>MAGAIKVGTWGGNGGSEWDMGPAYRIDSVKINAGDIIDAIEITFTRYGLTETQHYGGTGGEPHEIAFEDGEYIMSMEGHVVDYTGLTIIGK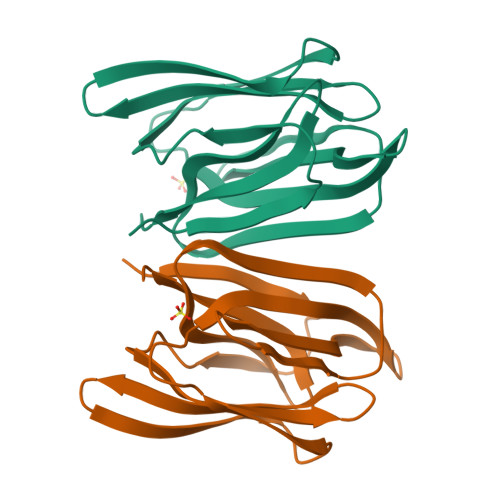LTLTTNRRTFGPFGAYEGTPFSIPVAEGKIAGFFGRAGSFIDAIGVYLMPNLEHHHHHH[16x]>[2x]GSHMASMLLDTFQGYNCYSSALGEYAKQKNI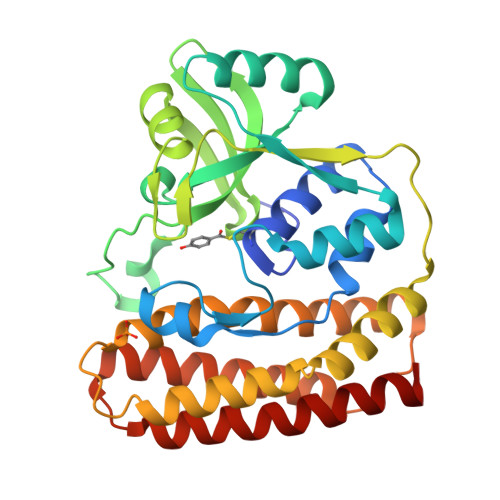DQVENIILSQWSFFFDEEQFYKNQWYTGAADGPVDVVLNEDLRNFANIEVLEHISSESQAIDEGRKVLEKHGLQIVLMDFYYMNSFNWKSLSRFNVTREHDPHFAVLTQINENSVHIIDPYYHHEENMSMEDFIKSRNSMTKQGKISFNSYEIFSNGTKKSNIKELLYYRFNRYLQEKMFGKITQFGQVVKKQLDNKDRKWAFTGYNCLNSVVYQHQNLINLQKKFSLEMPPNLQELLDNWALIRKKLFEYYSRGSYNTEEISNLICKVASSEEQFAQEVLKVL(~{Z})-3-[2-(naphthalen-2-ylmethyl)phenyl]-2-sulfanyl-prop-2-enoic 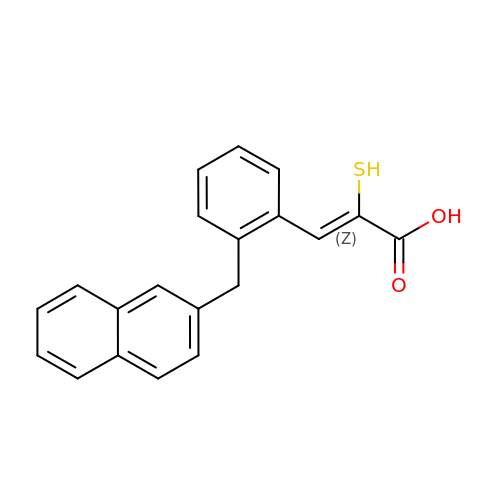acid | C20 H16 O2 S | LALSQKFPBIDRFB-UYRXBGFRSA-N The pilin subunits of GBS are assembled into high molecular weight polymers via a transpeptidation reaction catalyzed by specific pilin-associated class C sortases, through a common mechanism involving specific motifs present in the pilin proteins. The pilin-related sortases, which are integral membrane cysteine transpeptidases, cleave the LPXTG-like motif of the pilin proteins and, via the Thr residue, covalently join the C-terminus of one pilin subunit to a Lys side chain (ε amino group) on the next subunit. In this work, we present the high-resolution crystal structures of SrtC2 and SrtC1 from GBS PI-1.

The crystal structures of GBS SrtC1 and SrtC2 from PI-1 were determined at 1.87-Å and 1.8-Å resolution, respectively. The refined model of GBS SrtC1 includes residues 42–263 for chain A and 43–246 for chain B. The refined model of SrtC2 includes residues 56–236; the first N-terminal residues 41–55, and the C-terminal residues 237–256, were not visible in the electron density maps. Although SrtC1 crystallized as a dimer in the asymmetric unit, the dimer interface is only 615 Å2, suggesting it is not physiologically relevant. Analytical size-exclusion chromatography under near physiological conditions (pH 7.5, 75 mM NaCl) indicated that both enzymes are monomeric in solution, even at high (0.5–1 mM) concentration. GBS SrtC1 shows an identical arrangement of the catalytic pocket except for the Thr rotamer and the replacement of Phe86 with Tyr92. The lid residues 39–44 and 53–60 of SrtC1, and 89–95 of SrtC2, could not be modeled due to a lack of electron density, while the conserved residues of the DPX motif were well ordered in both structures. Unlike SrtA, GBS sortase C enzymes contain an additional N-terminal extension, composed of one (SrtC2) or two (SrtC1) α helices and a lid that blocks access of substrates to the active site. For both GBS SrtC1 and SrtC2 structures, the lid overlapped the LPAT peptide that is covalently bound to the catalytic Cys in the catalytic pocket of S. aureus SrtA. In particular, the conserved motif DPY or DPF in the SrtC lids overlap with the LPAT peptide, with the proline in a similar position in both the lid and the peptide. These observations suggest that the conserved residues in the lid that interact with the active site of GBS sortases are pseudo-substrates, insofar as they mimic the binding of the LPXTG motif in the catalytic site. However, SrtC1 showed the highest Vmax value for BP mimicking peptide (4.44×10−2 µM s−1) while SrtC2 for the AP1 peptide (2.60×10−2 µM s−1).

>ASHANINAFKEAVTKIDRVEINRRLELAYAYNASIAGAKTNGEYPALKDPYSAEQKQAGVVEYARMLEVKEQIGHVIIPRINQDIPIYAGSAEENLQRGVGHLEGTSLPVGGESTHAVLTAHRGLPTAKLFTNLDKVTVGDRFYIEHIGGKIAYQVDQIKVIAPDQLEDLYVIQGEDHVTLLTCTPYMINSHRLLVRGKRIPYVEKTVQKDSKTFRQQQYLT[2x]>[3x]MIHLYDAKSFAKLRAAQYAAFHTDAPGSWFDHTSGVLESVEDGTPVLAIGVESGDAIVFDKNAQRIVAYKEKSVKAED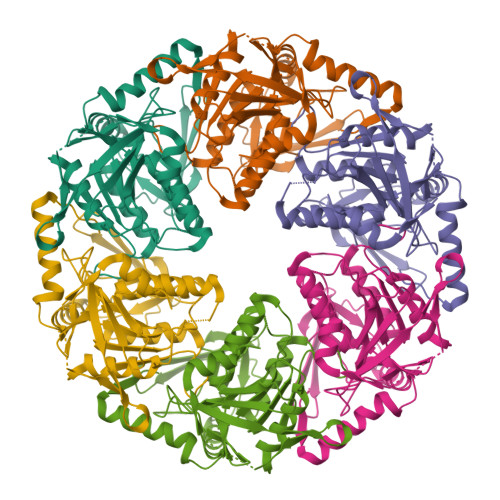GSVSVVQVENGFMKQGHRGWLVDLTGELVGCSPVVAEFGGHRYASGMVIVTGKGNSGKTPLVHALGEALGGKDKYATVRFGEPLSGYNTDFNVFVDDIARAMLQHRVIVIDSLKNVIGAAGGNTTSGGISRGAFDLLSDIGAMAASRGCVVIASLNPTSNDDKIVELVKEASRSNSTSLVISTDVDGEWQVLTRTGEGLARLTHTLQTSYGEHSVLTIHTSKQSGGKQASGKAIQTVIKNDELESVLRRLTSN2-methoxy-N-({6-[1-methyl-4-(methylamino)-1,6-dihydroimidazo[4,5-d]pyrrolo[2,3-b]pyridin-7-yl]pyridin-2-yl}methyl)acetamide | 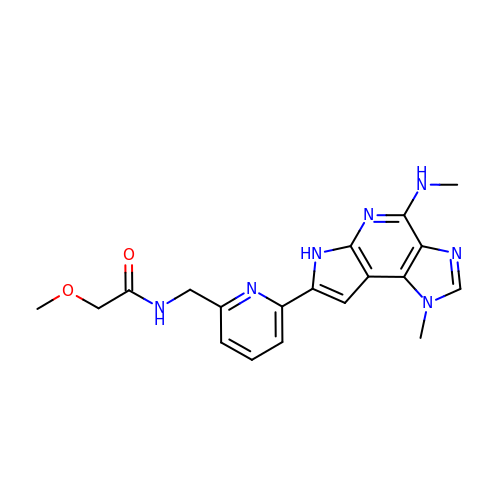C19 H21 N7 O2 | ULTCRVJUAZCGPP-UHFFFAOYSA-N>[8x]MTARPENPSTVHDFVGIGLGPFNLGLACLTEPIDELDGIFLESKPDFEWHAGMFLDGAHLQTPFMSDLVTLADPTSPYSFLNYLKEKGRLYSFYIRENFYPLRVEYDDYCRWAANKLSSIRFGTTVTEVRYEDD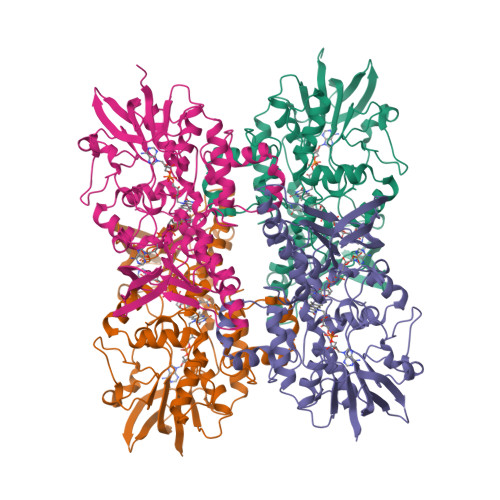LYVVTTSAGDVYRARHLVLGTGTPPYIPEACQGLDGDFIHNSRYVQHRSELVKKESITIVGSGQSAAEIYQDLLGEIDVHGYRLNWVTRSPRFFPLEYTKLTLEMTSPEYIDYYRELPEATRYRLTAEQKGLFKGIDGDLINEIFDLLYQKNLAGPVPTRLLTNSSLNSARHENGTYTLAFRQEEQGKDFEIESQGLVLATGYKYAEPEFLAPVKDRLVYDSQGNFDVSRAYAIDVTGRGVFLQNAGVHTHSITSPDLGMGAYRNSCIIRELLGTEYYPVEKTIAFQEFSV>[12x]MRIPFIQQKAAITPPAPSANPAKIFIRRLFNSGIAKSVVSYSNVMAAARAMEHPVVFRCLDKLGLTVQSVKWYVGADPDISGTGMSAKERKALQQVLNRPNSAMSGAQLRYAATLSWACFGRMAFKVSVMGDGSVNAIWPLGIPFLKQEFNKYGEVTTFQYGDEGNRE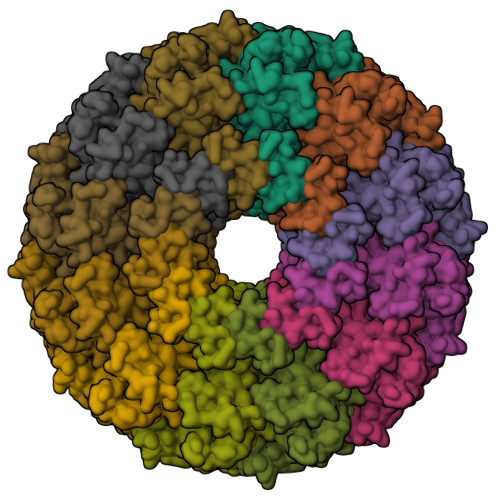SIKSFYSAAKNEKGRPIENYAFMIVKPSINGAMNLDVQNTPLQAVGMPVALYNGLMERALEQCDGTPNSKWFVTAGRDIGEVQSKEIKDGIDDTKPGGDSAGEIIFVFGEDVKLQEIKNDLSDIHSKIPLDDQARTIAGNFGIPIALLGFAAADGSKFASNYDESRKAFFEDTIEPGYLTPMEDGFSMFLCAPGSRVIFDRDSIPALKKSRADIAAVYEKVTFIDENEKREVTGWPKKEGQKPNDDA D-METHIONINE | C5 H11 N O2 S | 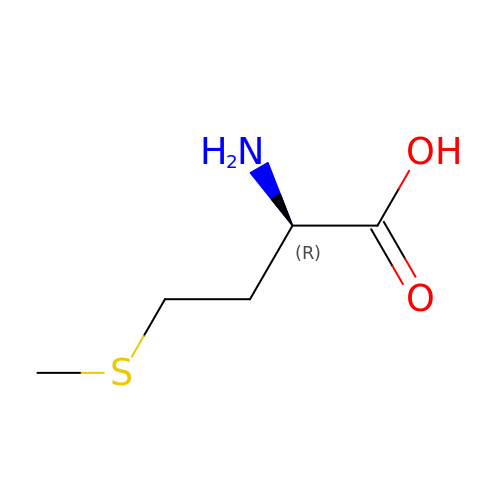FFEARJCKVFRZRR-SCSAIBSYSA-N> MDVSYLLDSLNDKQREAVAAPR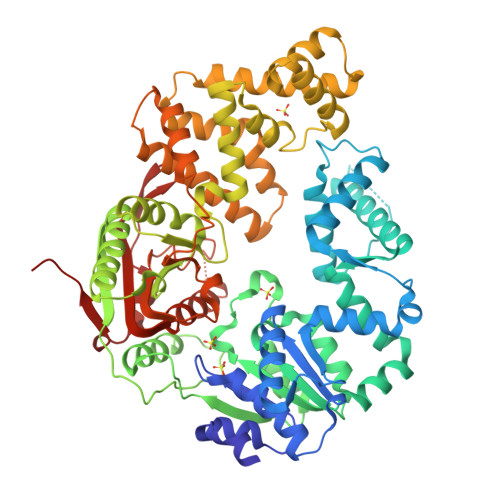SNLLVLAGAGSGKTRVLVHRIAWLMSVENCSPYSIMAVTFTNKAAAEMRHRIGQLMGTSQGGMWVGTFHGLAHRLLRAHHMDANLPQDFQILDSEDQLRLLKRLIKAMNLDEKQWPPRQAMWYINSQKDEGLRPHHIQSYGNPVEQTWQKVYQAYQEACDRAGLVDFAELLLRAHELWLNKPHILQHYRERFTNILVDEFQDTNNIQYAWIRLLAGDTGKVMIVGDDDQSIYGWRGAQVENIQRFLNDFPGAETIRLEQNYRSTSNILSAANALIENNNGRLGKKLWTDGADGEPISLYCAFNELDEARFVVNRIKTWQDNGGALAECAILYRSNAQSRVLEEALLQASMPYRIYGGMRFFERQEIKDALSYLRLIANRNDDAAFERVVNTPTRGIGDRTLDVVRQTSRDRQLTLWQACRELLQEKALAGRAASALQRFMELIDALAQETADMPLHVQTDRVIKDSGLRTMYEQEKGEKGQTRIENLEELVTATRQFSYNEEDEDLMPLQAFLSHAALEAGEGQADTWQDAVQLMTLHSAKGLEFPQVFIVGMEEGMFPSQMSLDEGGRLEEERRLAYVGVTRAMQKLTLTYAETRRLYGKEVYHRPSRFIGELPEECVEEVRLR2-[(1R)-1-(N-(3-METHYLBUTANOYL)-L-VALYL-L-ASPARAGINYL)-AMINO)-3-METHYLBUTYL]HYDROXYPHOSPHINYLOXY]-3-PHENYLPROPANOIC ACID METHYLESTER | C29 H47 N4 O9 P | 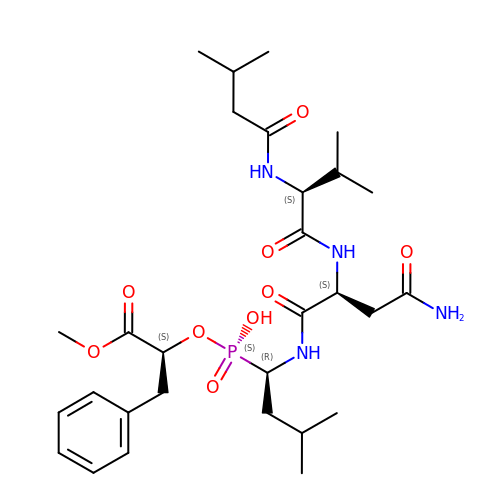SGKZZKPYLILTJX-RLBRRGQKSA-N> GAMAEKDF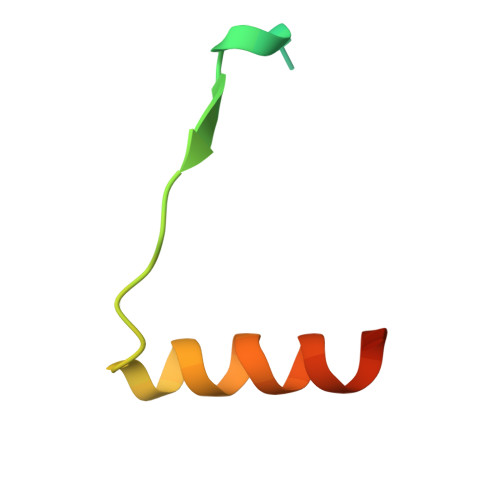KAIGKLTQEGSSMRTLEPVGPHFLAHARRVRHKRTFS>[24x]AKDCK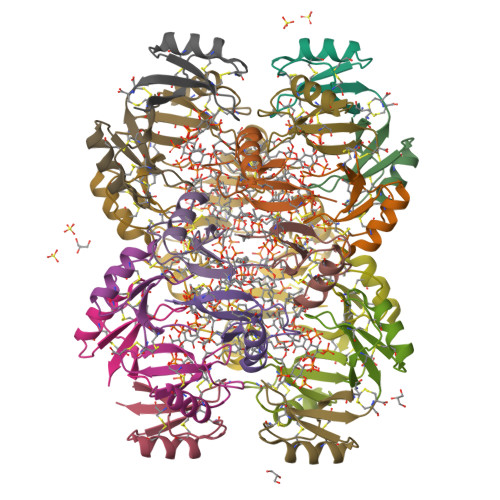RESNTFPGICITKPPCRKACIREKFTDGHCSKILRRCLCTKPC>[2x]GPLSLSVDAFKILEDPKWEFPRKNLVLGKTLGEGEFGKVVKATAFHLKGRAGYTTVAVKMLKENASPSELRDLLSEFNVLKQVNHPHVIKLYGACSQDGPLLLIMEYAKYGSLRGFLRESR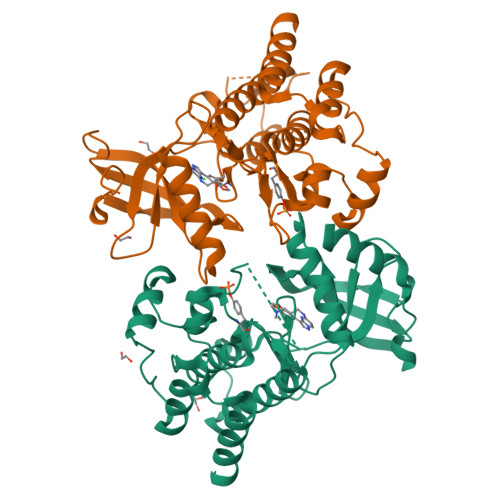KVGPGYLGSGGSRNSSSLDHPDERALTMGDLISFAWQISQGMQYLAEMKLVHRDLAARNILVAEGRKMKISDFGLSRDVYEEDSYVKRSQGRIPVKWMAIESLFDHIYTTQSDVWSFGVLLWEIVTLGGNPYPGIPPERLFNLLKTGHRMERPDNCSEEMYRLMLQCWKQEPDKRPVFADISKDLEKMMVKRR> AGVPFNTKYPYGPTSIADNQSEVTAMLKAEWEDWKSKRITSNGAGGYKRVQRDASTNYDTVSQGMGYGLLLAVCFNEQALFDDLYRYVKSHFNGNGLMHWHI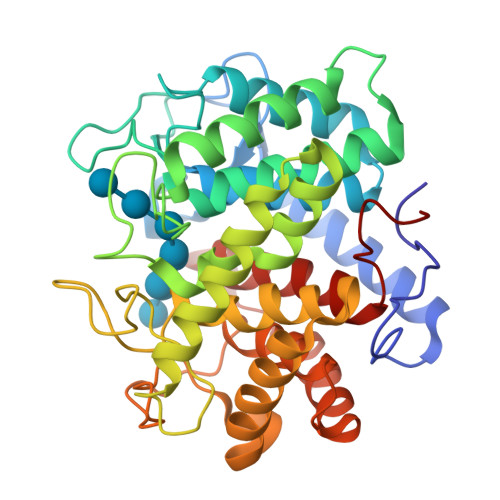DANNNVTSHDGGDGAATDADEDIALALIFADKLWGSSGAINYGQEARTLINNLYNHCVEHGSYVLKPGDRWGGSSVTNPSYFAPAWYKVYAQYTGDTRWNQVADKCYQIVEEVKKYNNGTGLVPDWCTASGTPASGQSYDYKYDATRYGWRTAVDYSWFGDQRAKANCDMLTKFFARDGAKGIVDGYTIQGSKISNNHNASFIGPVAAASMTGYDLNFAKELYRETVAVKDSEYYGYYGNSLRLLTLLYITGNFPNPLSDL> SNASSDKANGSGKAKDGGSLIIGVTGDPEVINPNYASDRVTLTIQQAVYAPLFWEVDGKPALAKSLDISDDNLTYTVKLKDGLTWHDGKPLTADDVVFTVNSILDTKQNSPNRGNFVFDDKPVKVEAVDDTTVKFTLPTVAPAFENTIKTFFPIPKHIFEGVENIEKSDKNKNPIGSGPYKFVEYKTGEYV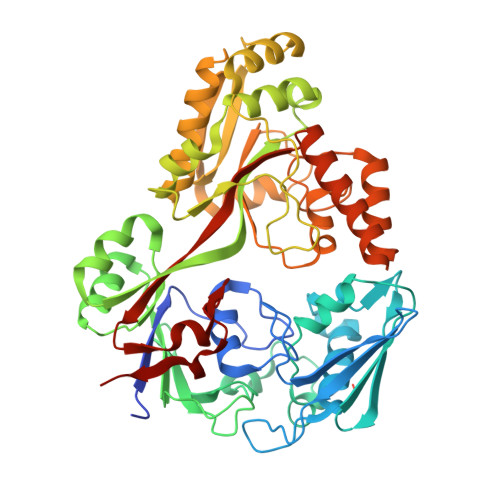SLERFNDYFDGKPKLDKVTFRITKDQNAANLALQNGEINLKSIQPSDRNKVEKASAVNIITYPENRLSYATFNENQPALKSKELRQALSYALDREEIIDAAYGSDEYAKPASSFLTENTKYFTDKVETYDQDIAKAKKLVKESGFDTSQKLTVYYLNNSKSQESIALYLQQQYKEIGVTLDLKPTDPNALSNITLDRKNADYSIALNGYIMGNDPDAYKSLYLSDAPYNYSNYHNKDLDALWEKGAVTADDKERQEIYEKIQNTIADDAVIYPISYDNAVLALDSRYGGQKAATPQPVTMFRDLSKLYLTE> SNVWLVGKTKASGAKAILLNGPQFGWFNPAYTYGIGLHGAGFNIVGNTPFAYPAILFGHNGHVSWGSTAGFGDGVDIFAEQVSPEDPNSYLHQGQWKKMLSRQETLNVKGEQPITFEIYRTVHGNVVKRDKTTHTAYSKARAWDGKE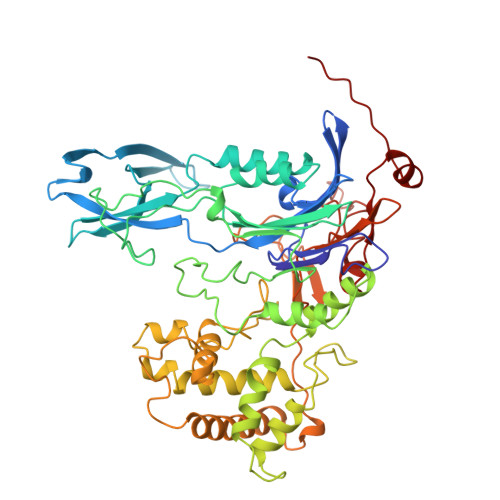LTSLMAWVKQGQAQNWQQWLDQAQNQALTINWYYADKDGNIGYVHTGHYPDRQINHDPRLPVSGTGEWDWKGIQPFANNPKVYNPKSGYIANWNNSPAKNYPASDLFAFLWGSADRVKEIDNRIEAYDKLTADDMWAILQQTSRVDLNHRLFTPFLTQATQGLPSNDNSVKLVSMLQQWDGINQLSSDGKHYIHPGSAILDIWLKEMLKATLGQTVPAPFDKWYLASGYETTQEGPTGSLNISTGAKLLYESLLEDKSPISQSIDLFSGQPQNDVIRKTLNTTYQKMIEKYGDNPANWQTPATALTFRENNFFGIPQALPQENFHQNEYHNRGTENDLIVFTEEGVSAWDVVAPGQSGFISPQGKPSPHYQDQLSLYQQFGKKPLWLNSEDVAPYIESTETLIIER>[4x]MAHHHHHHAKKRDHRLLGSNLQLFFFDSNVSPGSCFWLPAGARLYNKLMDFIRNEYRIREFTEVITPNIFSCDLWKTSGHYFAYKENMFIFDVEEKEWGLKPMNCPGHCVMFKHMNPSYRQLPIRLADFGVLHRNEFSGALNGLTRVRRFQQDDAHIFCTPEQIQEEVFKALDFLFFIYGQLGFTFDLFLSTMPKEHLGTE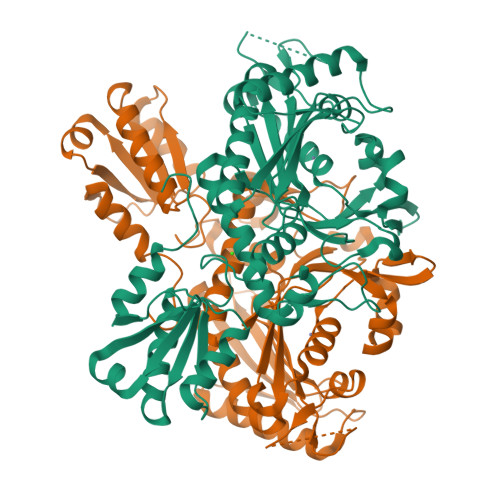EQWKEAENALKSALDKTGRDWKLNPGDGAFYGPKIDIMLWDALKRQHQCGTIQLDFQLPIRFNLQYRTDENISEESTNQEQPPSHQNADQNPDNSLKQGYRRPVIIHRAILGSVERMSAVILEHTGGKLPFWLSPRQAIVLSISEKTVEYAKSVERELCRRGFDVSGDYSAATINKKIRESQLLQWNYMLVIGENEARDKKVTLRCRDTTIPQELLTLDQLILKFSSMGFPSSIDSNSSNQ(1S,2R,5S,8R,8aR)-5-[2-(4-tert-butylphenyl)ethyl]octahydroindolizine-1,2,8-triol 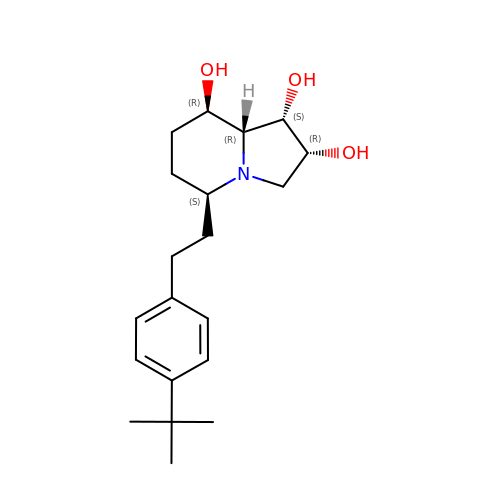| C20 H31 N O3 | QXPSLCODOUKVQZ-UURKPOQGSA-N>[2x]VFGSRNDRTLRRMRKVVNIINAMEPEMEKLSDEELKGKTAEFRARLEKGEVLENLIPEAFAVVREASKRVFGMRHFDVQLLGGMVLNERCIAEMRTGEGKTLTATLPAYLNALTGKGVHVVTVNDYLAQRDAENNRPLFEFLGLTVGINLPGMPAPAKREAYAADITYGTNNEYGFDYLRDNMAFSPEERVQRKLHYALVDEVDSILIDEARTPLIISGPAEDSSEMYKRVNKIIPHL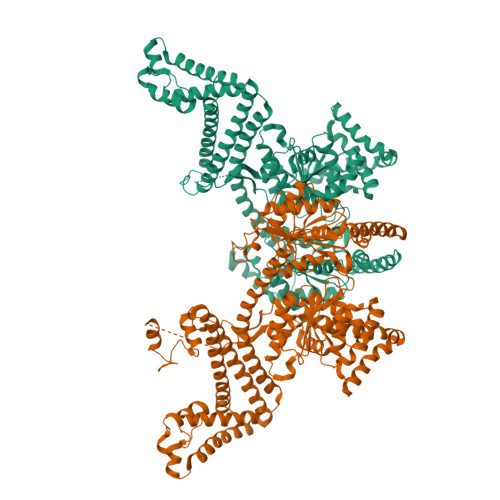IRQEKEDSETFQGEGHFSVDEKSRQVNLTERGLVLIEELLVKEGIMDEGESLYSPANIMLMHHVTAALRAHALFTRDVDYIVKDGEVIIVDEHTGRTMQGRRWSDGLHQAVEAKEGVQIQNENQTLASITFQNYFRLYEKLAGMTGTADTEAFEFSSIYKLDTVVVPTNRPMIRKDLPDLVYMTEAEKIQAIIEDIKERTAKGQPVLVGTISIEKSELVSNELTKAGIKHNVLNAKFHANEAAIVAQAGYPAAVTIATNMAGRGTDIVLGGSWQAEVAALENPTAEQIEKIKADWQVRHDAVLEAGGLHIIGTERHESRRIDNQLRGRSGRQGDAGSSRFYLSMEDALMRIFASDRVSGMMRKLGMKPGEAIEHPWVTKAIANAQRKVESRNFDIRKQLLEYDDVANDQRRAIYSQRNELLDVSDVSETINSIREDVFKATIDAYIPPQSLEEMWDIPGLQERLKNDFDLDLPIAEWLDKEPELHEETLRERILAQSIEVYQRKEEVVGAEMMRHFEKGVMLQTLDSLWKEHLAAMDYLRQGIHLRGYAQKDPKQEYKRESFSMFAAMLESLKYEVISTLSKVQVRMPEEVEELEQQRRMEAERLAQMQQLSHQD> NAMAIHVGIIDQDPVRLVTPLLDHRTVSRHIIFIGDHTQTVIYQRLSDVLNKRNISTDFFEIPAGSNTSAIKSAIRELAETLKARGEEVKFNASCGLRHRLLSAYEVFRSYHWPIFVVEPNSDCLCWLYPEGNNDTQVQDRITIADYLTIFGARGEFNEHQLSPQLDQQLYQLGERWASNALELGPGLATLNYLATTCRKEQKLDVELSDKQQGYRELNLLLSDLVEAKIASYENGILTFINEEARRFANGEWLETLVHSTVKQIQDDMPTIQDRSLNVQVYRQL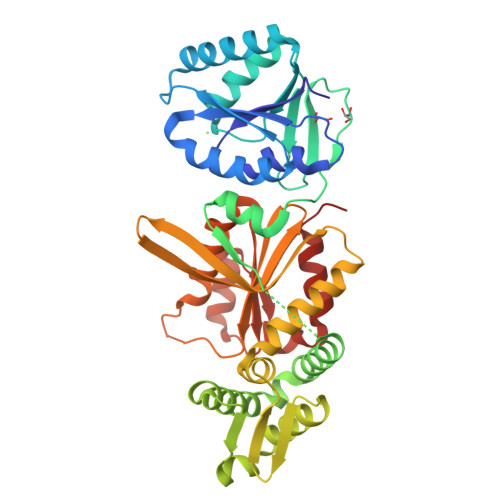GEREVRNELDVATVVNNKLHIIECKTKGMRDDGDDTLYKLESLRDLLGGLQARAMLVSFRPLRHNDITRAEDLGLALIGPDELKDLKTHLTQWFKAAGGN> HHHHHHGMPTLEMPV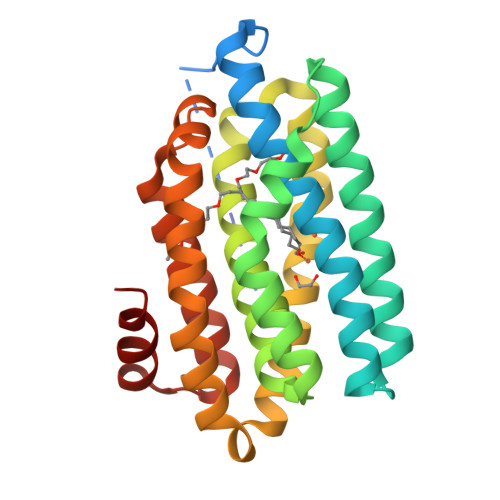AAVLDSTVGSSEALPDFTSDRYKDAYSRINAIVIEGEQEAHDNYIAIGTLLPDHVEELKRLAKMEMRHKKGFTACGKNLGVKADMDFAREFFAPLRDNFQTALGQGKTPTCLLIQALLIEAFAISAYHTYIPVSDPFARKITEGVVKDEYTHLNYGEAWLKANLESCREELLEANRENLPLIRRMADQVAGDAAVLQMDKEDLIEDFLIAYQESLTEIGFNTREITRMAAAALVS> MSSLQRASVSFNKPGHIPFGAVQGYAPGGVPAYSNKHDHYFSGERNIEDNIFFGFKYQCVEFARRWLLVRKGLLLPDVNWACHIFQLKEVRDAATTESFAVLQVRNGTTTKPEADALLVYPSTDANPVGHVGTITEVGDDYVCVADQNYRFHKWESSCAYKLKLDHRDGIWTIIDDIDADEIEIPLGWLTFPGRANRPEGAPPVALHPSLHFKEPPKPYLLRRNFLPTESKANWLDMNNPAERLFVEEFGMDVSRTRLEEKVVSYYESNHEFHLRCVAYGTQLHAIFMEATAQVIESDEKLRLFAIPEEFWPRIRHSWKYQQTYISGRFDFAFNNETGEVKCFEYNADSASTLLECGLIQQKWAESVGLDKQDTRGSGFAVERNLKMAWANSGATGRVHFCVDEEREEQYTALYCMQAAEAVGLEGKLCILFDEFRFDDNGHVVDSDGVRVRNVWKTWMWESAITDYYAAREERGENWKPSPK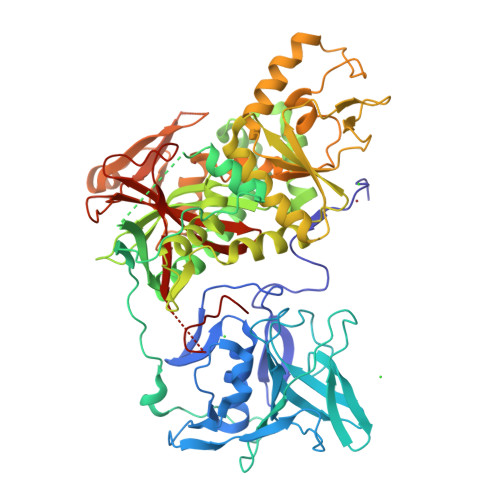DKVRLCDLLLGDDWEILYFEPMWKVIPSNKAILPMIYHNHPEHPAILKAEYELTDELRKHGYAKKPIVGRVGSNVIITSGDGVVHAESGGKYGKRNMIYQQLFELKKQDDYYAIIGGWMIGDAFSGTGIREDKSVITGVDSPFAAVRIKTDKLPHPVTLKDIDKMAEDE> MIESKTYAVLGLGNGGHAFAAYLALKGQSVLAWDIDAQRIKEIQDRGAIIAEGPGLAGTAHPDLLTSDIGLAVKDADVILIVVPAIHHASIAANIASYISEGQLIILNPGATGGALEFRKILRENGAPEVTIGETSSMLFTCRSERPGQVTVNAIKGAMDFACLPAAKAGWALEQIGSVLPQYVAVENVLHTSLT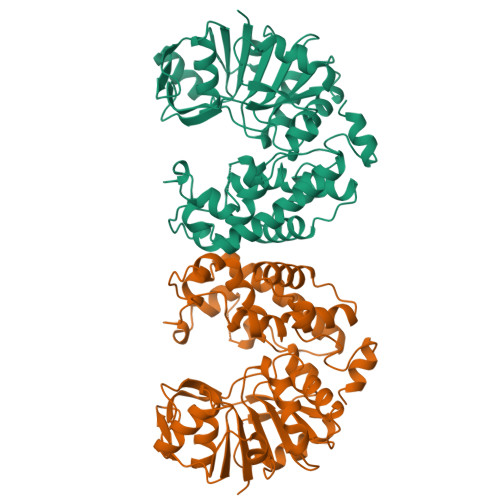NVNAVMHPLPTLLNAARCESGTPFQYYLEGITPSVGSLAEKVDAERIAIAKAFDLNVPSVCEWYKESYGQSPATIYEAVQGNPAYRGIAGPINLNTRYFFEDVSTGLVPLSELGRAVNVPTPLIDAVLDLISSLIDTDFRKEGRTLEKLGLSGLTAAGIRSAVE> VADGQQAYTLTLTAVDSEGNPVTGEASRLRLVPQDTNGVTVGAISEIKPGVYSATVSSTRAGNVVVRAFSEQYQLGTLQQTLKFVAGPLDAAHSSITLNPDKPVVGGTVTAIWTAKDANDNPVTGLNPDAPSLSGAAAAGSTASGWTDNGDGTWTAQISLGTTAGELDVMPKLNGQDAAANAAKVTVVADALSSNQSKVSVAEDHVKAGESTTVTLVAKDAHGNAISGLSLSASLTGTASEGATVSSWTEKGDGSYVATLTTGGKTGELRVMPLFNGQPAATEAAQLTVIAGEMSSANSTLVADNKTPTVKTTTELTFTMKDAYGNPVTGLKPDAPVFSGAASTGSERPSAGNWTEKGNGVYVSTLTLGSAAGQLSVMPRVNGQNAVAQP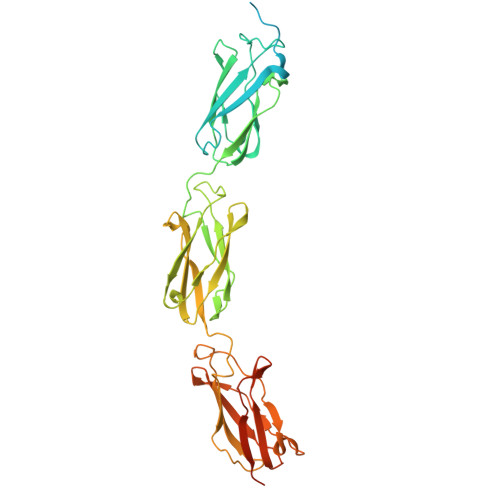LVLNVAGDASKAEIRDMTVKVNNQHHHHHH>ETGQLKHHHHHHEFTTDTDQACSIRDPNSGFVFNLNPLNSSQGYNVSGIGKIFMFNV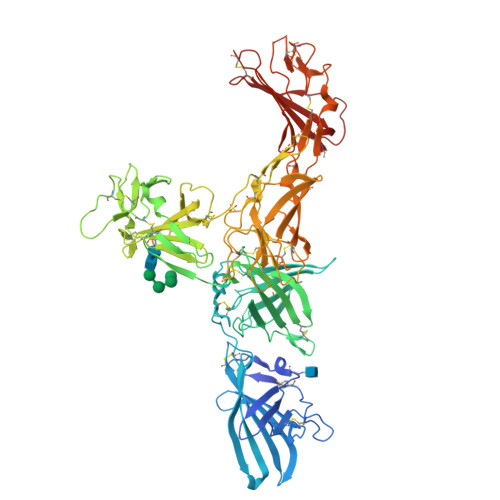CGTMPVCGTILGKPASGCEAETQTEELKNWKPARPVGIEKSLQLSTEGFITLTYKGPLSAKGTADAFIVRFVCNDDVYSGPLKFLHQDIDSGQGIRNTYFEFETALACVPSPVDCQVTDLAGNEYDLTGLSTVRKPWTAVDTSVDGRKRTFYLSVCNPLPYIPGCQGSAVGSCLVSEGNSWNLGVVQMSPQAAANGSLSIMYVNGDKCGNQRFSTRITFECAQISGSPAFQLQDGCEYVFIWRTVEACPVVRVEGDNCEVKDPRHGNLYDLKPLGLNDTIVSAGEYTYYFRVCGKLSSDVCPTSDKSKVVSSCQEKREPQGFHKVAGLLTQKLTYENGLLKMNFTGGDTCHKVYQRSTAIFFYCDRGTQRPVFLKETSDCSYLFEWRTQYACPPFDLTECSFKDGAGNSFDLSSLSRYSDNWEAITGTGDPEHYLINVCKSLAPQAGTEPCPPEAAACLLGGSKPVNLGRVRDGPQWRDGIIVLKYVDGDLCPDGIRKKSTTIRFTCSESQVNSRPMFISAVEDCEYTFAWPTATACPMKSNEHDDCQVTNPSTGHLFDLSSLSGRAGFTAAYSEKGLVYMSICGENENCPPGVGACFGQTRISVGKANKRLRYVDQVLQLVYKDGSPCPSKSGLSYKSVISFVCRPEAGPTNRPMLISLDKQTCTLFFSWHTPLACEQA[2x]> MAGSGSERAEHQIILPESHLSSPLVKHKLLYYWKLTGLPLPDECDFDHLILSRQWKKILESSTPDIERMIKLGRSVHQTLSHSSKLTGILHPRCLEDLVGLDIPDSTNKFRRIEKKIQIHNTRYGEPFTRLCSYVEKKLLGSSWTHKIRRSEEFDSLRTDPAFWFHSSWSTAKFAWLHVKQIQRHLIVAARTRSASNKLVTLSHRSGQVFITPELVIVTHTNENKFTCLSQELVLMYADMMEGRDMVNIISSTAVHLRCLAEKIDDILRLVDALARDLGNQVYDVVALMEGFAYGAVQLLEPSGTFAGDFFSFNLQELRDTLICLLPQRIADSVTHAIANIFSGLEQNQAAEMLCLLRLWGHPLLESRAAAKAVRAQMCAPKMVDFDMILQVLSFFKGTIINGYRKKNAGVWPRVKAHTIYGNVIAQLHADSAEISHDIMLREYKNLSAIEFEACIEYDPVTNLSMFLKDKAIAHPRNNWLASFRRNLLSEEQKKNVQDSTSTNRLLIEFLESNDFDPYKEMEYLTTLEYLRDDSVAVSYSLKEEEVKVNGRIFAKLTKKLRNCQVMAEGILADQIAPFFQGNGVIQDSISLTKSMLAMSQLSYNSNRKRITDCKERVSSSRNHDLKGKHRRRVATFITTDLQKYCLNWRYQTIKLFAHAINQLMGLPHFFEWIHLRLMDTTMFVGDPFNPPSDPTDYDLTKVPNDDIYIVSARGGIEGLCQKLWTMISIAAIQLAAARSHCRVACMVQGDNQVIAVTREVRPDDSPESVLTQLHEASDNFFRELIHVNHLIGHNLKDRETIRSDTFFIYSKRIFKDGAILSQVLKNSSKLVLVSGDLSENTVMSCANISSTVARLCENGLPKDFCYYLNYLMSCIQTYFDSEFSITSSTQSGSNQSWINDIPFIHSYVLTPAQLGGLSNLQYSRLYTRNIGDPGTTAFAEVKRLEAVGLLGPNIMTNILTRPPGNGDWASLCNDPYSFNFESVASPSIVLKKHTQRVLFETCSNPLLSGVHTEDNEAEEKALAEYLLNQEVIHPRVAHAIMEASSVGRRKQIQGLVDTTNTVIKIALSRKPLGIKRLARIINYSSMHAMLFRDDVFLSNRANHPLVSSDMCSLALADYARNRSWSPLTGGRKILGVSNPDTIELVEGEILSISGGCSKCDSGDEQFTWFHLPSNIELTDDTSKNPPMRVPYLGSKTQERRAASLAKIAHMSPHVKAALRASSVLIWAYGDNDINWTAALKLARSRCNISSEYLRLLSPLPTAGNLQHRLDDGITQMTFTPASLYRVSPYVHISNDSQRLFTEEGVKEGNVVYQQIMLLGLSLIESLFPMTVTKTYDEITLHLHSKFSCCIREAPVAVPFELTGVAPDLRVVASNKFMYDPNPVAEGDFARLDLAIFKSYELNLESYSTVELMNILSISSGKLIGQSVVSYDEETSIKNDAIIVYDNTRNWISEAQNSDVVRLFEYAALEVLLDCSYQLYYLRVRGLNNVVLYMSDLYKNMPGILLSNIAATISHPIIHSRLHTVGLISHDGSHQLADTDFIELSAKLLVSCTRRVVSGLYAGNKYDLLFPSVLDDNLNEKMLQLISRLCCLYTVLFATTREIPKIRGLPAEEKCAMLTEYLLSDAVRPLLSPEQVDSITSPSIVTFPANLYYMSRKSLNLIREREDRDSILALMFPQEPLFEFPLVQDIGARVKDQLTMKPAAFLHELDLSAPARYDAYTLEQARSDCALADMGEDQLVRYLFRGVGTASSSWYKASHLLSVPEIRCARHGNSLYLAEGSGAIMSLLELHIPHETIYYNTLFSNEMNPPQRHFGPTPTQFLNSVVYRNLQAEVPCKDGFVQEFRTLWRENTEESDLTSDKAVGYITSVVPYRSVSLLHCDIEIPPGSNQSLLDQLATNLSLIAMHSVREGGVVIVKILYSMGYYFHLLVNLFTPCSVKGYVLSNGYACRGDMECYVVFVMGYLGGPTFVNEVVRMAKTLIQRHGTLLAKSDETALMALFTSQKQRVDNILSSPLPRLAKLLRRNIDTALIEAGGQPVRPFCAESLVNTLSDITQTTQVIASHIDTVIRSVIYMEAEGDLADTVFLFTPYNLSIDGKKRTSLKQCTRQILEVTILGLGPEDLNRVGDIISLILRGTISLEDLIPLRTYLKMSTCPKYLKSV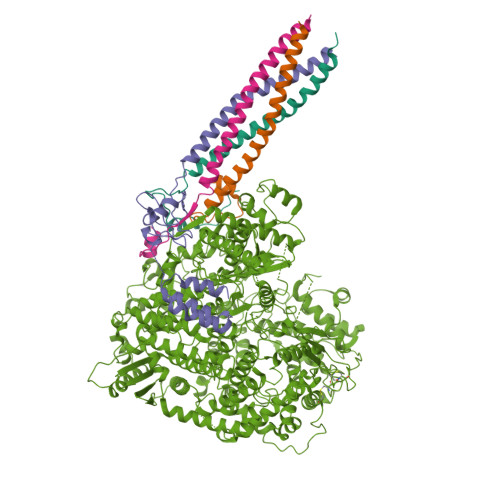LGLTKLREMFSDGSMLYLTRAQQKFYMKTVGNAVKGYYNSSKNENLYFQG;>MATFTDAEIDELFETSGTVIDSIITAQGKPVETVGRSAIPQGKTKALSLAWEKHGNTNTPAAQESAGEQDQHGQNQASNSNRATPEEGPHSSQAQAATQPQEDANESQLKTGASSSLLSMLDKLSNKSSNAKKGPPQSPPQQALHSKGSPAVEQTQHGANQGRAQQETGHQAAPSPGPPGTGVNIAFPGQRGVSPQSVGATQPAPQSGQNQGSTPASADHVQPPVDFVQAMMSMMEAISQRVSKIDYQLDLVLKQTSSIPTMRSEIQQLKTSVAVMEANLGMMKILDPGCANVSSLSDLRAVAKSHPVLIAGPGDPSPYVTQGGEIALNKLSQPVPHPSDLIKHATSGGPDIGIERDTVRALILSRPMHPSSSSKLLSKLDSAGSVEEIRKIKRLALNG[4x]>[2x]MKKVLLLFDIDGTLTPPRLSQPDEVREVIRRAKSAGFTVGTVGGSDLAKQIEQLGEDVFQQFDYVFAENGLLAYKHGKEIHRQNLLKELGNERIVKFVRR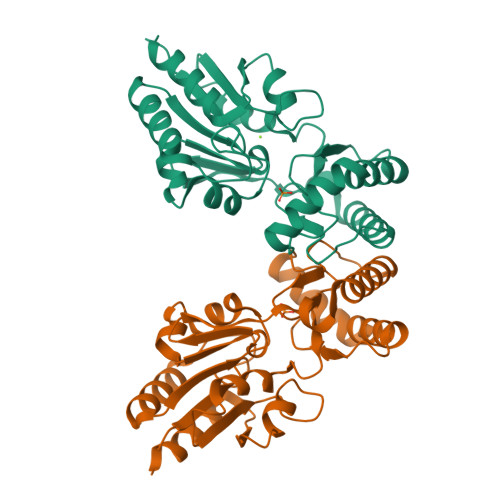ALRLLSELDIPVQRGTFIEYRNGMINVCPIGRNCTQSERDEFEVYDKEHHVREKLIKELQNSFPDYGLKYSIGGQISFDVFPVGWDKSYCLRFVENDFDEIHFFGDKTHAGGNDYEIYTDKRIIGHAVKSYKDTVDEVNKLISSK>[2x]SNAMTKVERLLINYKTLEEFK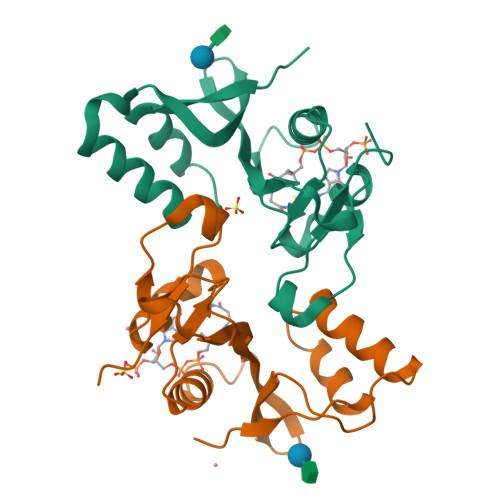KFKEYGIQELSMLEELQDNIIENDSTSPFYGIYFGDKLVARMSLYQVNGKSNPYFDNRQDYLELWKLEVLPGYQNRGYGRALVEFAKSFKMPIRTNPRMKSAEFWNKMNFKTVKYDMARDKGEDPLIWHPDMDREMTPGESA The serine-rich repeat (SRR) adhesins are a family of bacterial cell-surface glycoproteins containing two sequence motifs where serine constitutes ∼50% of the sequence. The binding region from S. sanguinis strain SK1 (residues 252–660 and termed SK1BR) differs from structurally characterized Siglec-containing binding regions in two ways. First, it contains two copies of the Siglec and Unique domains in tandem (SK1Siglec1-SK1Unique1-SK1Siglec2-SK1Unique2) with sequence identity/similarity of 39%/56% between the two Siglec domains and 44%/50% between the two Unique domains. The second way that SK1BR differs from other structurally characterized Siglec-like binding regions is that each of the putative Siglec domains of SK1BR contains a noncanonical YTRY sialic acid–binding sequence motif that lacks the central Thr-Arg deemed to be critical for binding in other Siglec-like adhesins.

We therefore determined cocrystal structures of SK1BR soaked with either 10 mm sialyl T-antigen (sTa), a core 1 glycan that can be conjugated to Ser or Thr residues of glycoproteins, or 10 mm 3´-sialyl-N-acetyllactosamine (3´sLn), a trisaccharide that can be a component of larger, branched glycans. For both sTa and 3´sLn, we observed the appearance of unambiguous electron density adjacent to the noncanonical YTRY motif of both SK1Siglec1 and SK1Siglec2. Thus, SK1Siglec1 and SK1Siglec2 are both capable of binding sialoglycan ligands and can do so simultaneously. SK1Siglec1 hydrogen-bonds to the sialic acid and galactose of both sTa and 3´sLn via the YTKY sequence. Here, the low temperature factors of sTa and SK1Siglec1 suggest that the ligand has little mobility when bound, which may be interpreted as strong binding. Consistent with the crystallographic temperature factor analysis, SK1Siglec1+Unique1 showed a statistically significant preference for sTa. Upon ligand binding, the temperature factors of all loops become more similar to the temperature factors of the Siglec domain core in both SK1Siglec1 and SK1Siglec2 (compare A and B with C–F). Moreover, the temperature factors of the YTKY motif in SK1Siglec1 decreased upon ligand binding (compare A, and E). The temperature factors of the YTFK motif in SK1Siglec2 decrease upon sTa binding but do not decrease upon 3´sLn binding (compare Fig. 8, compare B, D, and F).

>[2x]TDTTPPTITLPQEVIAYRGEEFEFFVETTDDSGRVNRVIVRNIEGADNSTYLDPNWIRYSTDNLSVPGNATPANPLRTRVYGIVPINHGVGPGDRYTKYVRAEDAAGNITALVDKQSERFVLVIRPQTEKYTPQVPTLTYVQNANSLTQTDKDAVIAAVKSANPNLPATSTYSVSENGTVTITYPDGSTDTIAAAQTVDTDRVAPVFVDEGRDYIFYRGEEGTAELHFYDNSGKITNVNFAGDLAASSTYNTLLGLGFTFNTPNINNPNNATEQNPLVTTIRGTIPKSLPAGPGGKYTFKVRATDASGLTSEAKIFRIVFANQTDKYTPNNPGSLTGVLNPQQLSTSEKTAIEEKVRAANTGNLPNNVQYVVNNDGSVTVIYPDDTPASRSRDTITADRTVQDLRPRNS ALPHA-N-DICHLOROACETYL-P-AMINOPHENYLSERINOL | C11 H14 Cl2 N2 O3 | 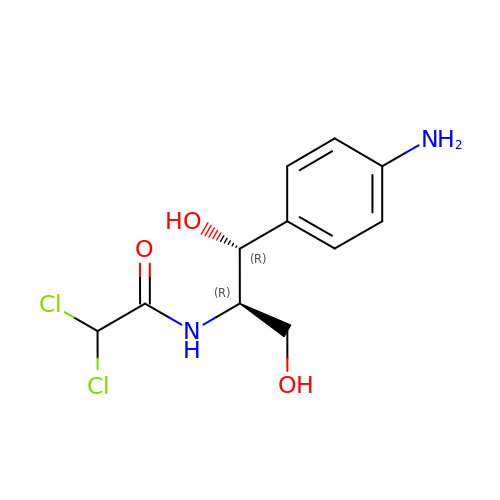BFLNGKUCFYKCFZ-RKDXNWHRSA-N> MLRITPSRYASKVTAGNAKNQAGSPRQKAKLFHVIPGTPVTPVEKLKEQRRRFGQDRYSRQPEYRPGRNVRMDPNTFTLYATTKGVMTIRTSRINPSYKWLDVEPDIQKVYRSRCMRAALQARGKASMMVAGNVHYRAELD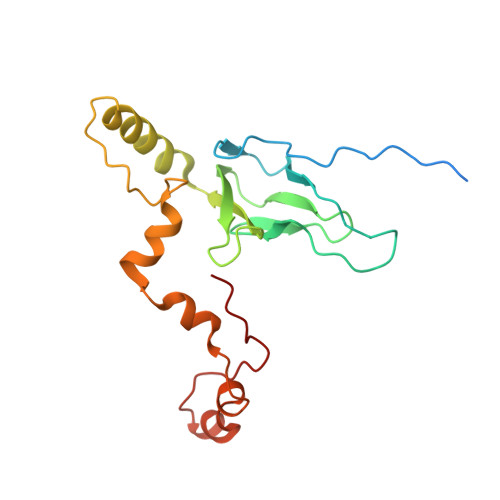HVTEPHWRERVMRVPKATERFQDPNYFTRGLVPSLRPLSRYSYE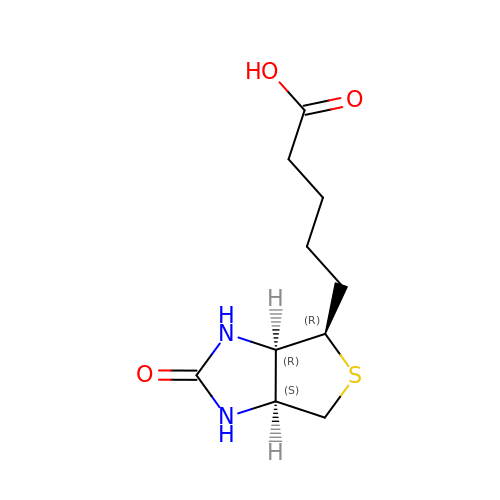5-[(3aR,4R,6aS)-2-oxohexahydro-1H-thieno[3,4-d]imidazol-4-yl]pentanoic acid | C10 H16 N2 O3 S | YBJHBAHKTGYVGT-ZXFLCMHBSA-N> GEIEFIESSKDAGFPVINTPSKTKLEPSVFHQVFEGNKEPAVLRSGDPRLKANFEEAIFSKYIGNVNTHVDEYMLEAVDHYAGQLATLDISTEPMKLEDAVYGTEGLEALDLTTSAGYPYVALGIKKRDILSKKTKDLTKLKECMDKYGLN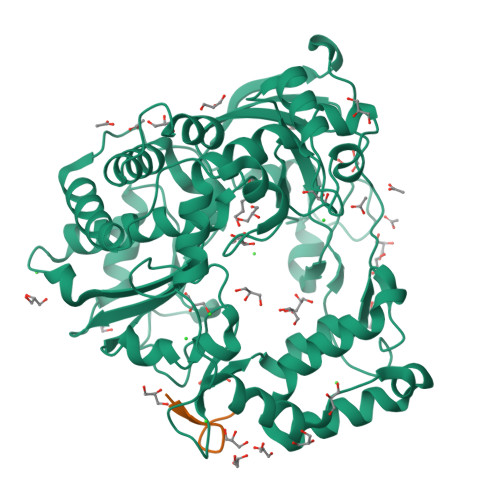LPMVTYVKDELRSIEKVAKGKSRLIEASSLNDSVAMRQTFGNLYKTFHLNPGVVTGSAVGCDPDLFWSKIPVMLDGHLIAFDYSGYDASLSPVWFACLKMLLEKLGYTHKETNYIDYLCNSHHLYRDKHYFVRGGMPSGCSGTSIFNSMINNIIIRTLMLKVYKGIDLDQFRMIAYGDDVIASYPWPIDASLLAEAGKGYGLIMTPADKGECFNEVTWTNATFLKRYFRADEQYPFLVHPVMPMKDIHESIRWTKDPKNTQDHVRSLCLLAWHNGEHEYEEFIRKIRSVPVGRCLTLPAFSTLRRKWLDSFHHHHHH;> GAYTGVPNQKPRVPTLRQAKVQ> LVHVASVEKGRSYEDFQKVYNAIALKLREDDEYDNYIGYGPVLVRLAWHISGTWDKHDNTGGSYGGTYRFKKEFNDPSNAGLQNGFKFLEPIHKEFPWISSGDLFSLGGVTAVQEMQGPKIPWRCGRVDTPEDTTPDNGRLPDADKDAGYVRTFFQRLNMNDREV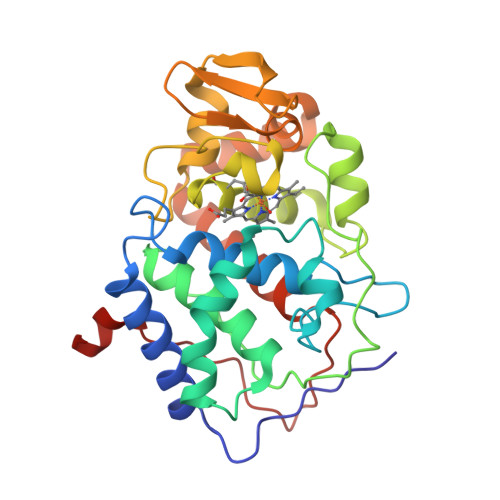VALKGAHALGKTHLKNSGYEGPWGAANNVFTNEFYLNLLNEDWKLEKNDANNEQWDSKSGYMMLPTDYSLIQDPKYLSIVKEYANDQDKFFKDFSKAFEKLLENGITFPKDAPSPFIFKTLEEQGL> 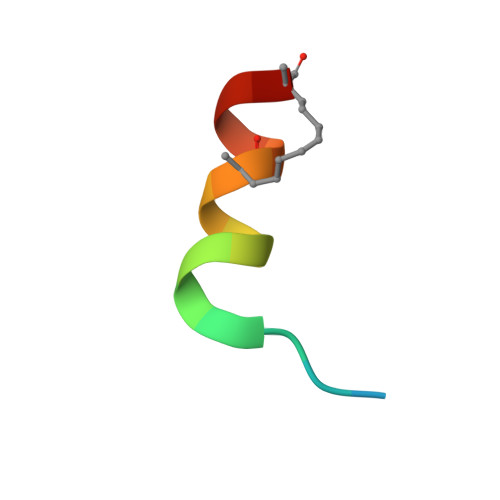XKKRYSREQLLLFQRLX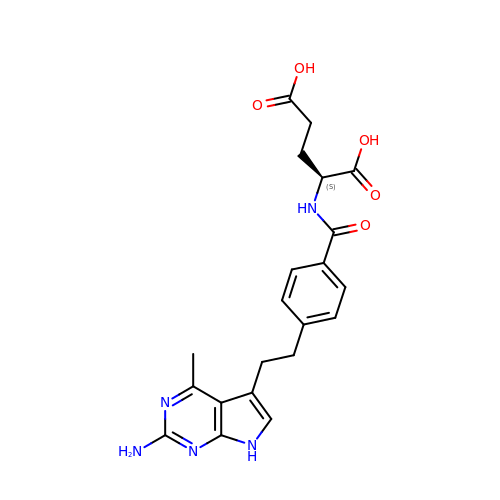N-[4-[2-(2-AMINO-4-METHYL-7H-PYRROLO[2,3-D]PYRIMIDIN-5-YL)-ETHYL]-BENZOYL]GLUTAMIC ACID | C21 H23 N5 O5 | FICRNCFTTZHHPO-HNNXBMFYSA-N> REFTIDFSTQQSYVSSLNSIRTEISTPLEHISQ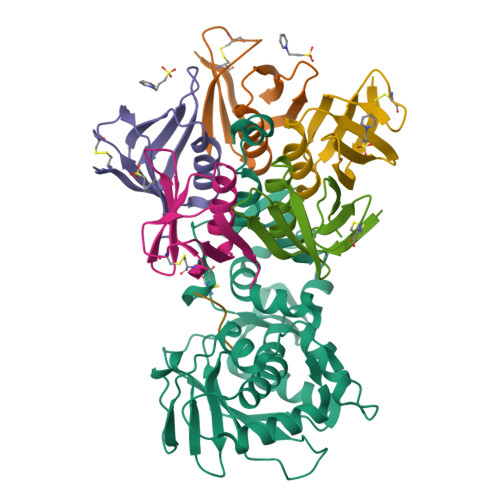GTTSVSVINHTPPGSYFAVDIRGLDVYQARFDHLRLIIEQNNLYVAGFVNTATNTFYRFSDFTHISVPGVTTVSMTTDSSYTTLQRVAALERSGMQISRHSLVSSYLALMEFSGNTMTRDASRAVLRFVTVTAEALRFRQIQREFRQALSETAPVYTMTPGDVDLTLNWGRISNVLPEYRGEDGVRVGRISFNNISAILGTVAVILNCHHQGARSVRAVNEESQPECQITGDRPVIKINNTLWESNTAAAFLNRKSQFLYTTGK;>[5x]ADCAKGKIEFSKYNEDDTFTVKVDGKEYWTSRWNLQPLLQSAQLTGMTVTIKSSTCESGSGFAEVQFNND;> RRRRAX> MPFVNKQFNYKDPVNGVDIAYIKIPNAGQMQPVKAFKIHNKIWV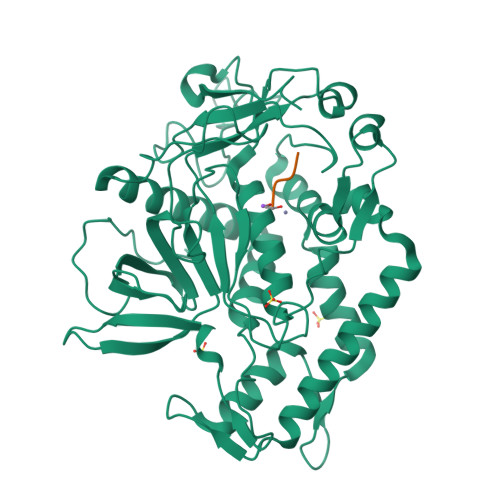IPERDTFTNPEEGDLNPPPEAKQVPVSYYDSTYLSTDNEKDNYLKGVTKLFERIYSTDLGRMLLTSIVRGIPFWGGSTIDTELKVIDTNCINVIQPDGSYRSEELNLVIIGPSADIIQFECKSFGHEVLNLTRNGYGSTQYIRFSPDFTFGFEESLEVDTNPLLGAGKFATDPAVTLAHELIHAGHRLYGIAINPNRVFKVNTNAYYEMSGLEVSFEELRTFGGHDAKFIDSLQENEFRLYYYNKFKDIASTLNKAKSIVGTTASLQYMKNVFKEKYLLSEDTSGKFSVDKLKFDKLYKMLTEIYTEDNFVKFFKVLNRKTYLNFDKAVFKINIVPKVNYTIYDGFNLRNTNLAANFNGQNTEINNMNFTKLKNFTGLFEHHHHHH;> CRGCX> ETGDSKPVFIKVPEDQTGLSGGVASFVCQATGEPKPRITWMKKGKKVSSQRFEVIEFDDGAGSVLRIQPLRVQRDEAIYECTATNSLGEINTSAKLSVLEEEQLPPGFP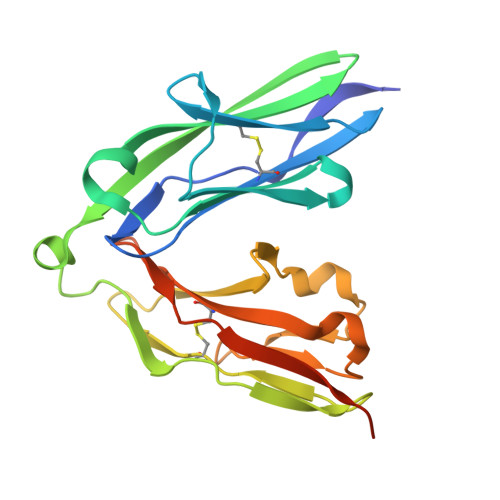SIDMGPQLKVVEKARTATMLCAAGGNPDPEISWFKDFLPVDPATSNGRIKQLRSGALQIESSEESDQGKYECVATNSAGTRYSAPANLYVRVRRVAGTKHHHHHH> MTQELGNANFENFI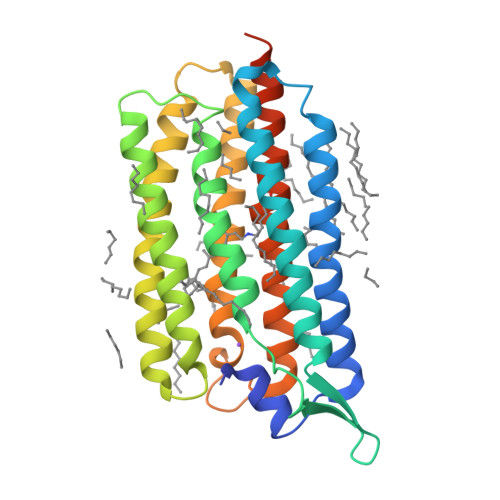GATEGFSEIAYQFTSHILTLGYAVMLAGLLYFILTIKNVDKKFQMSNILSAVVMVSAFLLLYAQAQNWTSSFTFNEEVGRYFLDPSGDLFNNGYRYLNWLIDVPMLLFQILFVVSLTTSKFSSVRNQFWFSGAMMIITGYIGQFYEVSNLTAFLVWGAISSAFFFHILWVMKKVINEGKEGISPAGQKILSNIWILFLISWTLYPGAYLMPYLTGVDGFLYSEDGVMARQLVYTIADVSSKVIYGVLLGNLAITLSKNKELENLYFQSGSHHHHHH>MQHWLDKLTDLAAIEGDECILKTGLADIADHFGFTGYAYLHIQHRHITAVTNYHRQWQSTYFDKKFEALDPVVKRARSRKHIFTWSGEHERPTLSKDERAFYDHASDFGIRSGITIPIKTANGFMSMFTMASDKPVIDLDREIDAVAAAATIGQIHARISFLRTTPTAEDAAWLDPKEATYLRWIAVGKTMEEIADVEGVKYNSVRVKLREAMK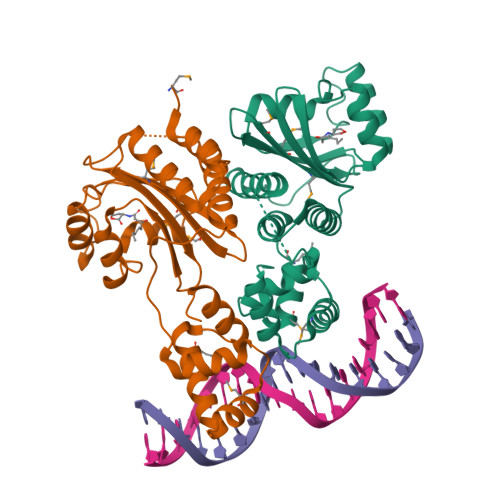RFDVRSKAHLTALAIRRKLI[4x]>MDYKDDDDKLVDSLRACVFDAYGTLLDVHSAVMRNADEVGASAEALSMLWRQRQLEYSWTRTLMHQYADFWQLTDEALTFALRTYHLEDRKGLKDRLMSAYKELSAYPDAAETLEKLKSAGYIVAILSNGNDEMLQAALKASKLDRVLD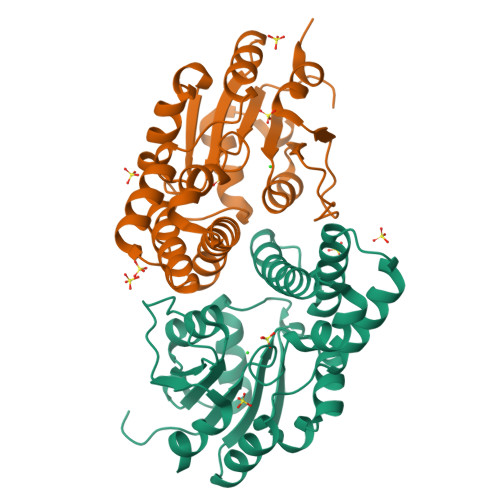SCLSADDLKIYKPDPRIYQFACDRLGVNPNEVCFVSSNAWDLGGAGKFGFNTVRINRQGNPPEYEFAPLKHQVNSLSELWPLLAKNVTKAA[2x]>[6x]TVYFHEEFKSMEHWTTSKHRDDFGKVEISAGKFYADAEKSKGLRLTEDARFYALSTAFPTPINNEKKSLVVSFSVKHEQDLKCGGGYIKLLPSMDPEKFHGETKYWLMFGPDRCGSQNRVHIILHYNGENREWSKRIRFPEDKLTHVYTLHIAADNSYEFFLDGESKAKGQLEEDWSLLLPREIVDGSGIPNPDFVEDSELHKVPEPLTHVGIDVWQVESGSIFKDIVIGDDLKEVLDLVEKTYGGLKKAEADALKVMEDMEKGDHHHHHH

Calreticulin (CRT) is a 46 kDa soluble multifunctional protein that was initially identified as an endoplasmic reticulum (ER) chaperone for monoglycosylated proteins and is also involved in Ca2+ regulation. Similar to its ER membrane homologue calnexin (CNX) ectodomain, CRT is composed of a globular domain, into which a flexible arm-like P (proline-rich) domain is inserted. The globular domain is made up of seven concave and six convex β-sheets forming a legume lectin fold. We have investigated the CRTs of two distinct parasites, Trypanosoma cruzi (TcCRT) and Entamoeba histolytica (EhCRT), for which a pathogenic role has been proposed.

T. cruzi is the causative agent of Chagas disease, an acute illness affecting 12 million people in Latin America and causing 50 000 deaths per year. Cell-surface expression of TcCRT only occurs in its infective trypomastigote stage, where it has been proposed to enhance host-cell infection and mother-to-child transmission. Several trials were required to define a suitable TcCRT construct because simultaneously removing these flexible areas drastically reduced the molecular solubility and stability, as checked for example by fluorescent spectroscopy (not shown). The diffraction quality of these crystals was slightly improved by adding a large amount (1 M) of glucose (Glc) to the crystallization droplet. A similar EhCRT construct was then produced and beautiful crystals were obtained. The X-ray structures of the corresponding TcCRT and EhCRT constructs were solved using molecular replacement and refined to 2.45 and 2.15 Å resolution, respectively. The first evidence is now provided of a complex conformational transition with the junction reoriented towards P-domain closure. SAXS experiments also provided additional information about the flexibility of T. cruzi CRT in solution, thus complementing crystallographic data on the open conformation. SAXS was used to study the overall shape and flexibility of several TcCRT constructs. The TcCRT SAXS analysis above suggests that the junction domain is stable in the solution structures.GCN5-related N-acetyltransferase (GNAT) toxin, with an acetyltransferase activity-dependent mechanism of translation inhibition, represents a relatively new and expanding family of type II TA toxins. We here describe a group of GNAT-Xre TA modules widely distributed among Pseudomonas species. Notably, other than arresting translation through acetylating aminoacyl-tRNAs, PacT can directly bind to Fur, a key ferric uptake regulator, to attenuate its DNA-binding affinity and thus permit the expression of downstream iron-acquisition-related genes. Previously studies on GNAT-RHH TA family also observed pronounced growth arrest after expression of the GNAT-type toxin and co-expression of its upstream antitoxin gene counteracted the toxic effect. It has been also demonstrated that the translational repression function of GNAT-type toxin depend on its acetyltransferase activity which transfers the acetyl group from acetyl coenzyme A (AcCoA) to the amine group of aa-tRNAs, subsequently resulting in the inhibition of translation.

In addition, both the structures of PacT homologues from P. jinjuensis and P. flexibilis are in complex with AcCoA, and share similar fold with PacT in superposition (mean RMSD 0.28Å). Because GNAT-Xre toxins are widespread in Pseudomonas species, which also have highly conserved Fur proteins, we also tested the binding between GNAT toxins and Fur proteins from P. jinjuensis and P. flexibilis. Consistently, both PacT homologs could specifically bind to the DNA-binding domain of Fur. We also found that PacT homologs from other Pseudomonas species could bind to the Fur protein, suggesting that the direct PacT–Fur interaction is a common mechanism for PacT-type toxins. Based on these results, we conclude that the specific interactions between GNAT-Xre toxins and Fur proteins seem to be a common and novel bidirectional regulatory mechanism, indicating that Fur proteins play vital roles in bacterial iron uptake.

>[4x]MFKPQPVTLRRGALCLEPLAEADLVELLSLAEANRQSLIYMNGPLRPDWYRQGLAEQREGQAVIYAVRQDHALVGTTRFFDFMPGLPAVEIGGTWLAEDRHGSGLNAAIKFLMLRQAFEQWEMVRVQLKTAASNLRAQRAIEKLGARREGQLRNHRRLADGRLDDSILYSITDRDWPEIRRTLETELSAAARP> GSAQADFDIPAGPLAPALAHFGQSAHILLSYPTALTEGRSTSGLAGRFDIDQGLAILLAGTGLEASRGANASYSLQASASTG;> GAMGQDWRADYHSRIGEQRRLTLADGTQVQLNTDSALNVAFDQQARRLRLVRGEMLITRPALADSRPLWVDTEHGRLESTLAQFNVRLHGQHTQATVYQGSVALQPALHAYPPILLGAGEQASFNQQGLLARQAVAAVAPAWSQGMLVAQGQPLAAFIEDLARYRRGHLACDPALAGLRVSGTFPLENTDKIIAAVAETLQLEVQHFTRYWVTLKPRMA

Each of these homologous pathways involves a TonB-dependent transporter/transducer, an inner membrane sigma regulator, and an extra-cytoplasmic function sigma factor. Here, we report the 1.56 Å resolution X-ray crystal structure of the periplasmic domain of the CSS sigma regulator, PupR, in complex with the NTSD of the transducer, PupB, revealing a unique fold and topological arrangement of domains. The CCSSD comprises two subdomains: residues 110–238 that we call the C-terminal juxta-membrane subdomain (CJM) and residues 250–324, comprising a Secretin/TonB, short N-terminal subdomain (STN). The CJM has a novel-fold, whereas the STN is structurally homologous to the PupB NTSD.

The final Se-Met and native models include residues 111–323 of PupR, residues 49–128 PupB, 20 tartrate molecules, and 355 or 319 water molecules, respectively. The Se-Met and native proteins have practically identical structures, although there are some differences in interacting residues at the complex interface. The interface between the CCSSD and the NTSD has a substantial buried surface area of ∼1438.6 Å2 and involves residues from the linker, β17 and α2 of the CCSSD and α1 and β2 of the NTSD. The interface is stabilized by salt bridges between NTSD His72 and Glu83 to CCSSD Glu292 and Arg284, respectively, as well as an extensive hydrogen-bonding network. Hydrophobic interactions at the interface include two extensively buried residues, NTSD Leu74 (84% buried) and CCSSD Met251 (98% buried). Interestingly, a polar interaction linking NTSD His72 and CCSSD Glu292 is critical for interaction between the two proteins, but the atoms involved are variable. In the native crystal structure, the Nϵ2 of the His72 imidazole ring forms a salt bridge with Glu292 Oϵ1 and Oϵ2. The Glu292 side chain adopts a different conformer with the closest atom, Oϵ2, shifting 4.7 Å from His72. These results suggest that in addition to the complementary surfaces, a polar interaction at this position is critical to the interaction.> AVCPDGTRVSHAACCAFIPLAQDLQETIFQNECGEDAHEVIRLTFHDAIAISRSQGPKAGGGADGSMLLFPTVEPNFSANNGIDDSVNNLIPFMQKHNTISAADLVQFAGAVALSNCPGAPRLEFLAGRPNKTIAAVDGLIPEPQDSVTKILQRFEDAGGFTPFEVVSLLASHSVARADKVDQTIDAAPFDSTPFTFDTQVFLEVLLKGVGFPGSANNTGEVASPLPLGSGSDTGEMRLQSDFALAHDPRTACIWQGFVNEQAFMAASFRAAMSKL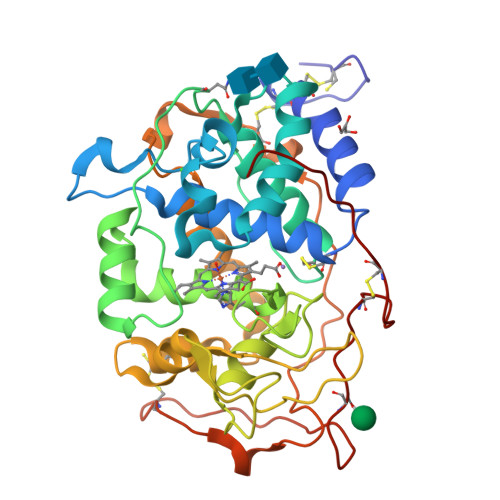AVLGHNRNSLIDCSDVVPVPKPATGQPAMFPASTGPQDLELSCPSERFPTLTTQPGASQSLIAHCPDGSMSCPGVQFNGPA>SRSFEQKHLAVVDAFFQTYHVKPDFIARSPGRVNLIGEHIDYCDFSVLPLAIDVDMLCAVKILDEKNPSITLTNADPKFAQRKFDLPLDGSYMAIDPSVSEWSNYFKCGLHVAHSYLKKIAPERFNNTPLVGAQIFCQSDIPTGGGLSSAFTCAAALATIRANMGKNFDISKKDLTRITAVAEHYVGVNNGGMDQATSVYGEEDHALYVEFRPKLKATPFKFPQLKNHEISFVIANTLVKSNKFETAPTNYNLRVIEVTVAANALATRYSVALPSHKDNSNSERGNLRDFMDAYYARYENQAQPWNGDIGTGIERLLK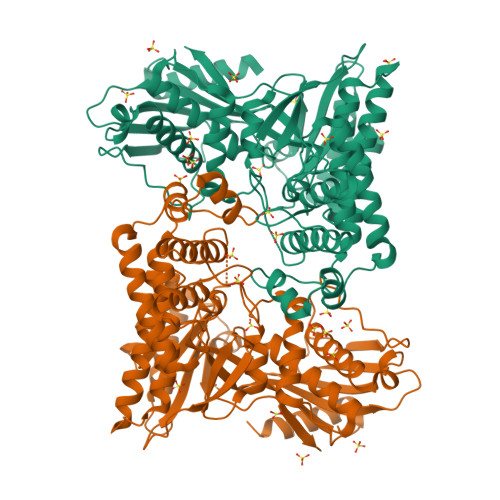MLQLVEESFSRKKSGFTVHEASTALNCSREEFTRDYLTTFPVRFQVLKLYQRAKHVYSESLRVLKALKMMTSATFHTDEDFFTDFGRLMNESQASCDKLYECSCIETNQICSIALANGSFGSRLTGAGWGGCTIHLVPSGANGNVEQVRKALIEKFYNVRYPDLTDEELKDAIIVSKPALGTCLYEQ[2x]> MKKSKRKNAQAQEAQ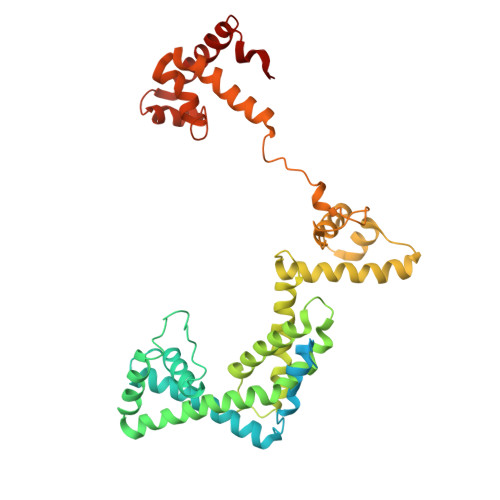ETEVLVQEEAEELPEFPEGEPDPDLEDPDLTLEDDLLDLPEEGEGLDLEEEEEDLPIPKISTSDPVRQYLHEIGQVPLLTLEEEVELARKVEEGMEAIKKLSEITGLDPDLIREVVRAKILGSARVRHIPGLKETLDPKTVEEIDQKLKSLPKEHKRYLHIAREGEAARQHLIEANLRLVVSIAKKYTGRGLSFLDLIQEGNQGLIRAVEKFEYKRRFKFSTYATWWIRQAINRAIADQARTIRIPVHMVETINKLSRTARQLQQELGREPTYEEIAEAMGPGWDAKRVEETLKIAQEPVSLETPIGDEKDSFYGDFIPDEHLPSPVDAATQSLLSEELEKALSKLSEREAMVLKLRKGLIDGREHTLEEVGAFFGVTRERIRQIENKALRKLKYHESRTRKLRDFLD>[9x]MSYNFTGTPTGEGTGGNSLTTDLNTQFDLANMGWIGVASAGVWIMVPGIGLLYSGLSRKKHALSLLWASMMASAVCIFQWFFWGYSLAFSHNTRGNGFIGTLEFFGFRNVLGAPSSVSSLPDILFAVYQGMFAAVTGALMLGGACERARLFPMMVFLFLWMTIVYCPIACWVWNAEGWLVKLGSLDYAGGLCVHLTSGHGGLVYALILGKRNDPVTRKGMPKYKPHSVTSVVLGTVF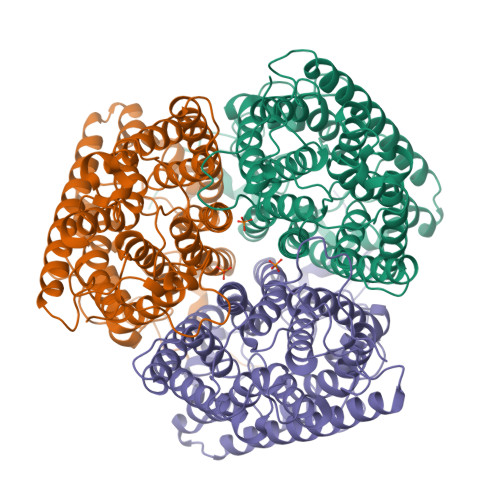LWFGWMFFNGGSAGNATIRAWYSIMSTNLAAACGGLTWMVIDYFRCGRKWTTVGLCSGIIAGLVGITPAAGFVPIWSAVVIGVVTGAGCNLAVDLKSLLRIDDGLDCYSIHGVGGCIGSVLTGIFAADYVNATAGSYISPIDGGWINHHYKQVGYQLAGICAALAWTVTVTSILLLTMNAIPFLKLRLSADEEELGTDAAQIGEFTYEESTAYIPEPIRSKTSAQMPPPHENIDDKIVGNTDAEKNSTPSDASSTKNTDHIVHHHHHH> MNLAEKMYKAGNAMYRKGQYTIAIIAYTLALLKDPNNAEAWYNLGNAAYKKGEYDEAIEAYQKALELDPNNAEAWYNLGNAYYKQGDYDEAIEYYQKALELDPNNAE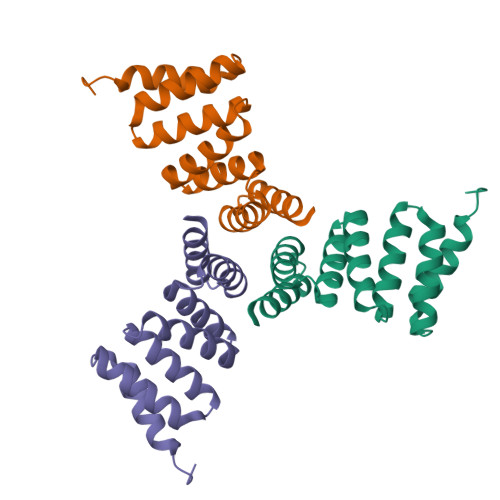AKQNLGNAKQKQGLEHHHHHH> XS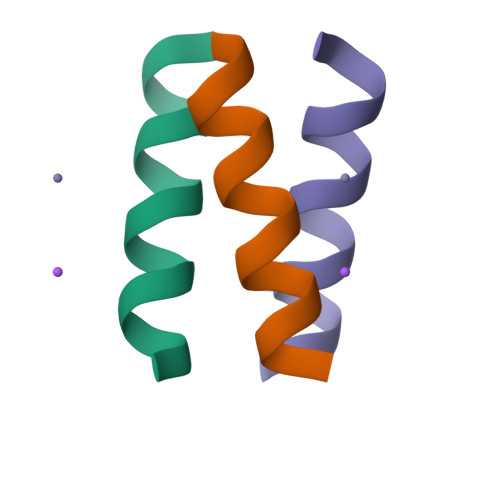IRELEARIRELELRIG>MSNYYYYYGGGRYDWLKTVEPTNFLKIGLPYQAHPLHLQHQATTPPSILEKFKRADILLNEVKAEMDPLMLQPETEKKLFQILSSIDMFKGLRKKVEFTYNAQIVTNAWLKMYELLNTMNFNNTSQAFCNC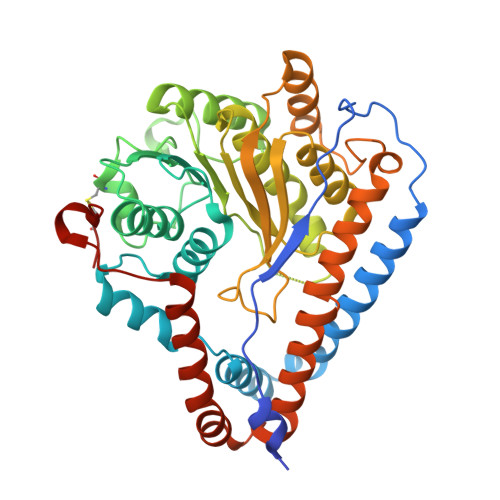ELPGGFISAINHFNYTMMHYPTFNWVASSLYPSSETDALEDHYGLYQCNPDNWLMQSPLLKKNIDYNNGDVTIASNVKNLALRATQRLTPIHLYTADGGINVGHDYNKQEELNLKLHFGQALTGLLSLSKGGNMILKHYTLNHAFTLSLICVFSHFFEELYITKPTSSRPTNSETYIVGKNRLRLFTPKEEQVLLKRLEFFNDTPLVDLSLYQNLLESVYFAVETIHLKQQIEFLNFGMKCYRHFYNKIKLLNDYLAPKKKIFQDRWRVLNKLYVLEKKHKLKLCASHHHHHH[2x]> MSSLRLVSSSTIQAANDNNDDSSQLIDLTVWDLIGLERESIQQGLLYHHPNQVDTPNQIQHLKHSLSSTLSFFPPFAGRLVITEYEDNTATCFIACNNAGALFVHAVAENTTISDILQPNKYVPPIVNSLFSLNGVKNREGTIQPLLVVQVTELVDGIFIGLTVNHVVADGKSFWLFVNSWAEISRGFQKPSKLPTLERWFLNDTDHPIRFSFSMEEEKKKFQSGQLTTRFFHFTRENIAHLKSKANGEVTLGNTERRISSLQALLAHVWRSVVRCERIDPQEVLYYILLIDARTRLIPPLEDDYFGNAGDAGVVIMKAGELLEGGLGNV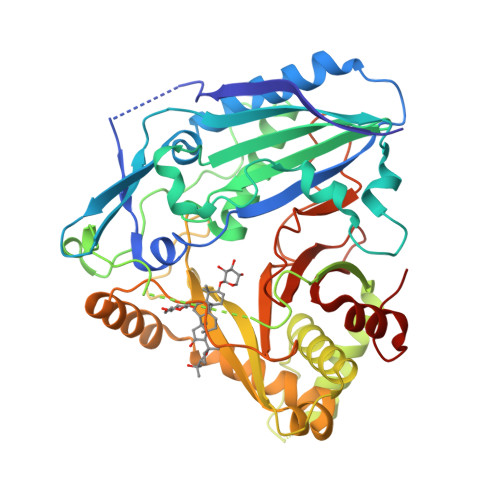AWNMNKVISLNSDEKIKNRYKSWLRTPQLPSMGMHTTFASQLLIIANSPRFNVYGNDFGWGKPLAVRSSAENKRDCKIVLFAGAEEGSIDIEVCLPYEILEALGNDAEFLDNHSIG> MGKKQRFSLRKYKSGTFSVLIGSVFLVMTTTVAADELSTMSEPTITNHAQQQAQHLTNTELSSAESKSQDTSQITPKTNREKEQSQDLVSEPTTTELADTDAASMANTGPDATQKSASLPPVNTDIHD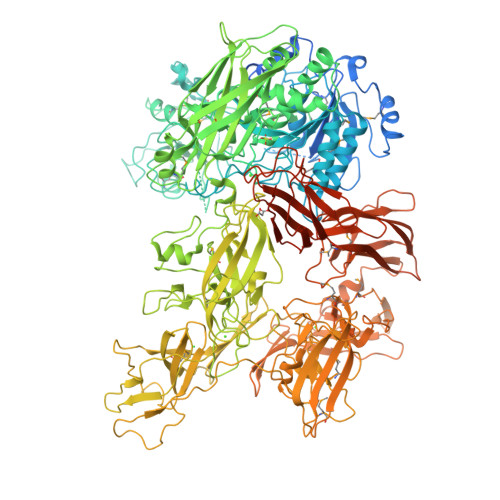WVKTKGAWDKGYKGQGKVVAVIDTGIDPAHQSMRISDVSTAKVKSKEDMLARQKAAGINYGSWINDKVVFAHNYVENSDNIKENQFEDFDEDWENFEFDAEAEPKAIKKHKIYRPQSTQAPKETVIKTEETDGSHDIDWTQTDDDTKYESHGMHVTGIVAGNSKEAAATGERFLGIAPEAQVMFMRVFANDVMGSAESLFIKAIEDAVALGADVINLSLGTANGAQLSGSKPLMEAIEKAKKAGVSVVVAAGNERVYGSDHDDPLATNPDYGLVGSPSTGRTPTSVAAINSKWVIQRLMTVEELEKRADLNHGKAIYSESVDFKNIKDSLGYDKSHQFAYVKESTDAGYNAQDVKGKIALIERDPNKTYDEMIALAKKHGALGVLIFNNKPGQSNRSMRLTANGMGIPSAFISHEFGKAMSQLNGNGTGSLEFDSVVSKAPSQKGNEMNHFSNWGLTSDGYLKPDITAPGGDIYSTYNDNHYGSQTGTSMASPQIAGASLLVKQYLEKTQPNLPKEKIADIVKNLLMSNAQIHVNPETKTTTSPRQQGAGLLNIDGAVTSGLYVTGKDNYGSISLGNITDTMTFDVTVHNLSNKDKTLRYDTELLTDHVDPQKGRFTLTSRSLKTYQGGEVTVPANGKVTVRVTMDVSQFTKELTKQMPNGYYLEGFVRFRDSQDDQLNRVNIPFVGFKGQFENLAVAEESIYRLKSQGKTGFYFDESGPKDDIYVGKHFTGLVTLGSETNVSTKTISDNGLHTLGTFKNADGKFILEKNAQGNPVLAISPNGDNNQDFAAFKGVFLRKYQGLKASVYHASDKEHKNPLWVSPESFKGDKNFNSDIRFAKSTTLLGTAFSGKSLTGAELPDGYYHYVVSYYPDVVGAKRQEMTFDMILDRQKPVLSQATFDPETNRFKPEPLKDRGLAGVRKDSVFYLERKDNKPYTVTINDSYKYVSVEDNKTFVERQADGSFILPLDKAKLGDFYYMVEDFAGNVAIAKLGDHLPQTLGKTPIKLKLTDGNYQTKETLKDNLEMTQSDTGLVTNQAQLAVVHRNQPQSQLTKMNQDFFISPNEDGNKDFVAFKGLENNVYNDLTVNVYAKDDHQKQTPIWSSQAGAGASAIESTAWYGITARGSKVMPGDYQYVVTYRDEHGKEHQKQYTISVNDKKPMITQGRFDTINGVDHFTPDKTKALGSSGIVREEVFYLAKKNGRKFDVTEGKDGITVSDNKVYIPKNPDGSYTISKRDGVTLSDYYYLVEDRAGNVSFATLRDLKAVGKDKAVVNFGLDLPVPEDKQIVNFTYLVRDADGKPIENLEYYNNSGNSLILPYGKYTVELLTYDTNAAKLESDKIVSFTLSADNNFQQVTFKMTMLATSQITAHFDHLLPEGSRVSLKTAQGQLIPLEQSLYVPKAYGKTVQEGTYEVVVSLPKGYRIEGNTKVNTLPNEVHELSLRLVKVGDASDSTGDHKVMSKNNSQALTASATPTKTTTPATAKALPSTGEKMGLKLRIVGLVLLGLTCVFSRKKSTKD> HMQHITVRLPKKARAMIVGEITNVFKDKYPIADKLKVIPEYDVIEQDLCKLLSPGFPKQPLRVYKFGSRITGIGNRSSDLDLFVDIGNTFHTFEHRASNATVAKLRAMRKFFCDSEDWRLINFIEQARVPIIKTCHLPTGIECDICLNSMGFCNTNLLKYIFESQPLTQYMCIYVKNWLERCKLTEQISTYSITLMVIYFLQLQALLPPIAMLQIEDAANQAVLVGPWVVNFAQKSFSELGLQQLKATVPVIKGFLRNFFAYFAKFDYEHFLVCPYIGQANVEIAKIERMLHARYSAYVSDNPECSIQLKKPMVVQDPIQLNHNVTKAVT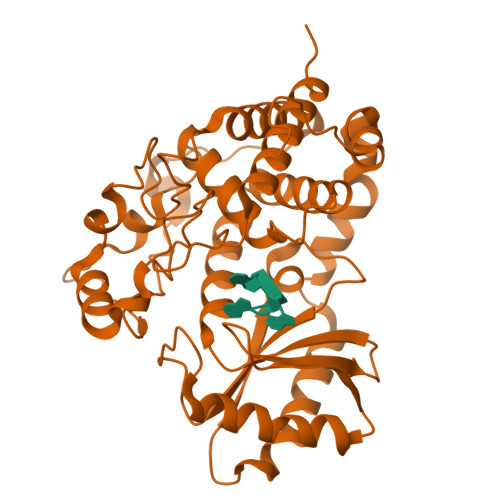KYGLQTFVDYCQQTAELLEEP> MLNFKGYQIEIELKDGKRITGTLKQVSPKSLTLTDAVFQDGGVSPVFKIKADKLYD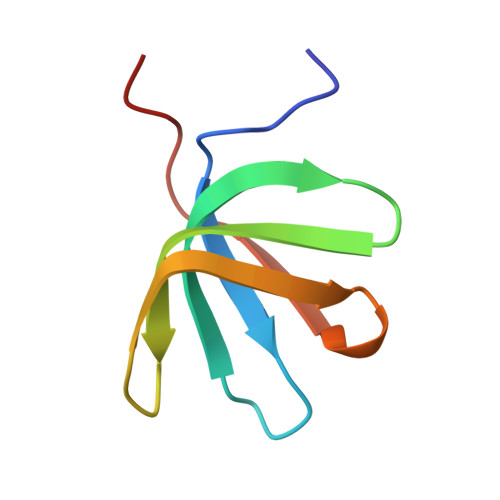LKVLKLPPNA> MAAQGFLLIATFLLVLMVLARPLGSGLARLINDIPLPGTTGVERVLFRALGVSDREMNWKQYLCAILGLNMLGLAVLFFMLLGQHYLPLNPQQLPGLSWDLALNTAVSFVTNTNWQSYSGETTLSYFSQMAGLTVQNFLSAASGIAVIFALIRAFTRQSMSTLGNAWV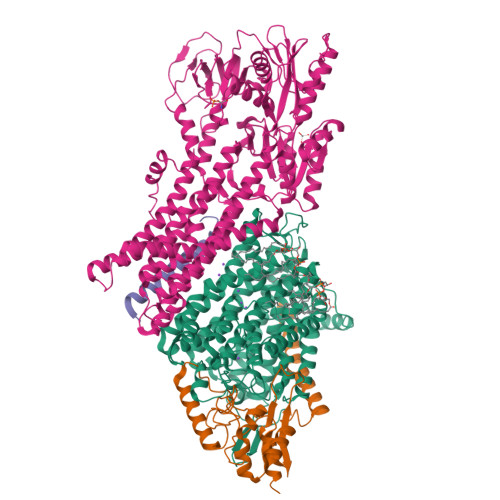DLLRITLWVLVPVALLIALFFIQQGALQNFLPYQAVNTVEGAQQLLPMGPVASQEAIKMLGTNGGGFFNANSSHPFENPTALTNFVQMLAIFLIPTALCFAFGEVMGDRRQGRMLLWAMSVIFVICVGVVMWAEVQGNPHLLALGTDSSINMEGKESRFGVLVSSLFAVVTTAASCGAVIAMHDSFTALGGMVPMWLMQIGEVVFGGVGSGLYGMMLFVLLAVFIAGLMIGRTPEYLGKKIDVREMKLTALAILVTPTLVLMGAALAMMTDAGRSAMLNPGPHGFSEVLYAVSSAANNNGSAFAGLSANSPFWNCLLAFCMFVGRFGVIIPVMAIAGSLVSKKSQAASSGTLPTHGPLFVGLLIGTVLLVGALTFIPALALGPVAEYLS;> MSRKQLALFEPTLVVQALKEAVKKLNPQAQWRNPVMFIVWIGSLLTTCISIAMASGAMPGNALFSAAISGWLWITVLFANFAEALAEGRSKAQANSLKGVKKTAFARKLREPKYGAAADKVPADQLRKGDIVLVEAGDIIPCDGEVIEGGASVDESAITGESAPVIRESGGDFASVTGGTRILSDWLVIECSVNPGETFLDRMIAMVEGAQRRKTPNEIALTILLIALTIVFLLATATLWPFSAWGGNAVSVTVLVALLVCLIPTTIGGLLSAIGVAGMSRMLGANVIATSGRAVEAAGDVDVLLLDKTGTITLGNRQASEFIPAQGVDEKTLADAAQLASLADETPEGRSIVILAKQRFNLRERDVQSLHATFVPFTAQSRMSGINIDNRMIRKGSVDAIRRHVEANGGHFPTDVDQKVDQVARQGATPLVVVEGSRVLGVIALKDIVKGGIKERFAQLRKMGIKTVMITGDNRLTAAAIAAEAGVDDFLAEATPEAKLALIRQYQAEGRLVAMTGDGTNDAPALAQADVAVAMNSGTQAAKEAGNMVDLDSNPTKLIEVVHIGKQMLMTRGSLTTFSIANDVAKYFAIIPAAFAATYPQLNALNIMCLHSPDSAILSAVIFNALIIVFLIPLALKGVSYKPLTASAMLRRNLWIYGLGGLLVPFIGIKVIDLLLTVCGLV;> MSGLRPALSTFIFLLLITGGVYPLLTTVLGQWWFPWQANGSLIREGDTVRGSALIGQNFTGNGYFHGRPSATAEMPYNPQASGGSNLAVSNPELDKLIAARVAALRAANPDASASVPVELVTASASGLDNNITPQAAAWQIPRVAKARNLSVEQLTQLIAKYSQQPLVKYIGQPVVNIVELNLALDKLDE;> MSAGVITGVLLVFLLLGYLVYALINAEAF> MLRKTPLFAMATTRKALVGNGPTFSTGGECMNTCDIQNAFPMNDRGVRSSSPFQEPNTAIYDSYLAWTYF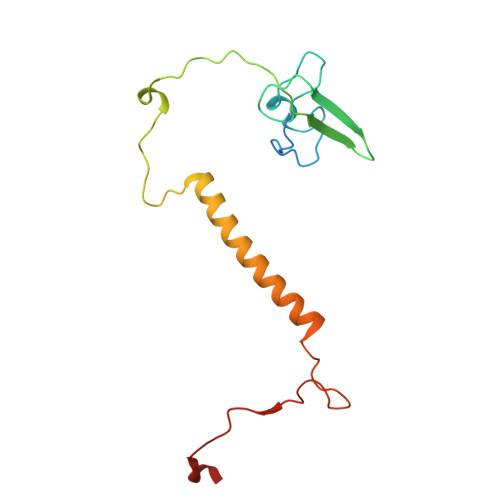QPMDVHIEKLPAPEAKYYQRHTKKPWDVSSTELTEIQSRKKYFQTLGYLVAFIYLYFLMPKEKSFSGLSGPDGHWIMLPKGRPELF>MHHHHHHMANRKLEKMASIDVHLRQLVPGKVSEDDKLVEYDALLLDRFLDILQDLHGEDLRETVQELYEHSAEYEGKHEPKKLEELGSVLTSLDPGDSIVIAKAFSHMLNLANLAEEVQIAYRRRIKKLKKGDFVDESSATTESDLEETFKKLVGDLNKSPEEIFDALKNQTVDLVLTAHPTQSVRRSLLQKHGRIRDCLAQLYAKDITPDDKQELDEALQREIQAAFRTDEIKRTPPTPQDEMRAGMSYFHETIWKGVPKFLRRVDTALKNIGIEERVPYNAPLIQFSSWMGGDRDGNPRVTPEVTRDVCLLARMMAATMYFNQIEDLMFEMSMWRCNDELRARADEVHANSRKDAAKHYIEFWKSIPTTEPYRVILGDVRDKLYHTRERAHQLLSNGHSDVPVEATFINLEQFLEPLELCYRSLCSCGDRPIADGSLLDFLRQVSTFGLSLVRLDIRQESDRHTDVLDAITTHLDIGSYREWSEERRQEWLLSELSGKRPLFGSDLPKTEEIADVLDTFHVIAELPADSFGAYIISMATAPSDVLAVELLQRECRVKQPLRVVPLFEKLADLEAAPAAVARLFSVDWYKNRINGKQEVMIGYSDSGKDAGRLSAAWQLYKAQEELVKVAKEYGVKLTMFHGRGGTVGRGGGPTHLVILSQPPDTINGSLRVTVQGEVIEQSFGEEHLCFRTLQRFTAATLEHGMRPPISPKPEWRALLDEMAVVATEEYRSVVFQEPRFVEYFRLATPELEYGRMNIGSRPSKRKPSGGIESLRAIPWIFAWTQTRFHLPVWLGFGSAIRHVIEKDVRNLHMLQDMYQHWPFFRVTIDLIEMVFAKGDPGIAALYDKLLVSEELWPFGEKLRANFEETKKLILQTAGHKDLLEGDPYLKQRLRLRDSYITTLNVCQAYTLKRIRDPSYHVTLRPHISKEIAESSKPAKELIELNPTSEYAPGLEDTLILTMKGIAAGLQNT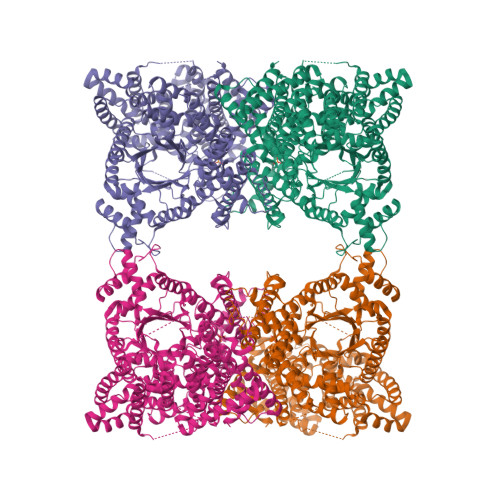G[2x]> GPLGSKIVRIEKARDIPLGATVRNEMDSVIISRIVKGGAA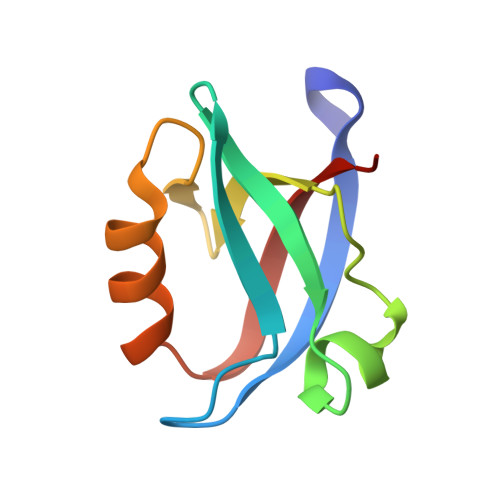EKSGLLHEGDEVLEINGIEIRGKDVNEVFDLLSDMHGTLTFVLIPSQ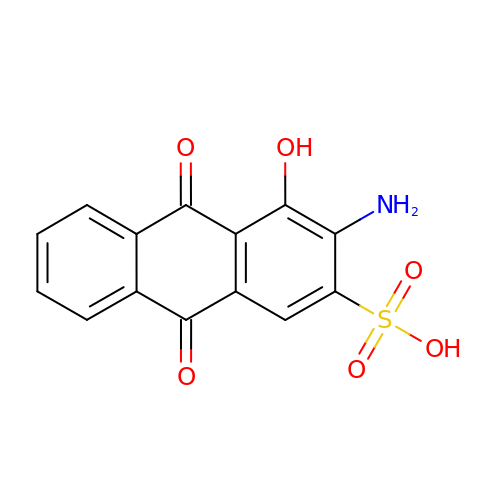3-amino-4-hydroxy-9,10-dioxo-9,10-dihydroanthracene-2-sulfonic acid | C14 H9 N O6 S | UJIPILVKRSZCAC-UHFFFAOYSA-N>[2x]AGITGTWYNQLGSTFIVTAGA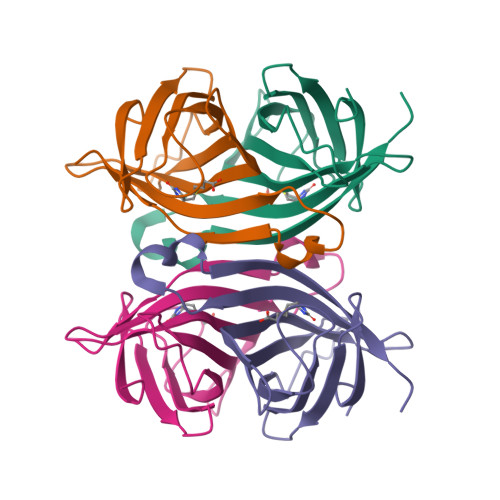DGALTGTYESAVGNAESRYVLTGRYDSAPATDGSGTALGWTVAWKNNYRNAHSATTWSGQYVGGAEARINTQWLLTSGTTEANAWKSTLVGHDTFTKVKP>[3x]MKTIKDRIAKWSAIGLLSAVAATAFYAPSASAHGEKSQAAFMRMRTIHWYDLSWSKEKVKINETVEIKGKFHVFEGWPETVDEPDVAFLNVGMPGPVFIRKESYIGGQLVPRSVRLEIGKTYDFRVVLKARRPGDWHVHTMMNVQGGGPIIGPGKWITVEGSMSEFRNPVTTLTGQTVDLENYNEGNTYFWHAFWFAIGVAWIGYWSRRPIFIPRLLMVDAGRADELVSATDRKVAMGFLAATILIVVMAMSSANSKYPITIPLQAGTMRGMKPLELPAPTVSVKVEDATYRVPGRAMRMKLTITNHGNSPIRLGEFYTASVRFLDSDVYKDTTGYPEDLLAEDGLSVSDNSPLAPGETRTVDVTASDAAWEVYRLSDIIYDPDSRFAGLLFFFDATGNRQVVQIDAPLIPSFM;>[3x]MSAAQSAVRSHAEAVQVSRTIDWMALFVVFFVIVGSYHIH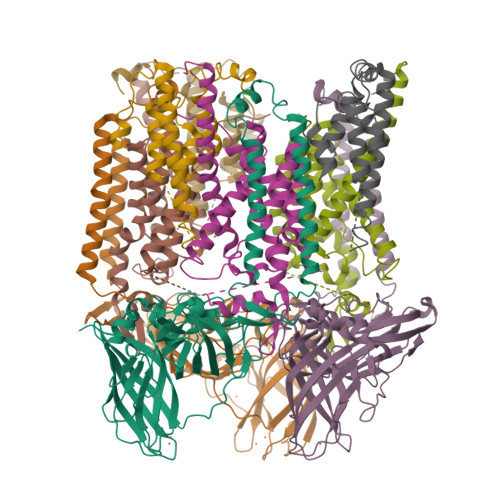AMLTMGDWDFWSDWKDRRLWVTVTPIVLVTFPAAVQSYLWERYRLPWGATVCVLGLLLGEWINRYFNFWGWTYFPINFVFPASLVPGAIILDTVLMLSGSYLFTAIVGAMGWGLIFYPGNWPIIAPLHVPVEYNGMLMSIADIQGYNYVRTGTPEYIRMVEKGTLRTFGKDVAPVSAFFSAFMSILIYFMWHFIGRWFSNERFLQST;>[3x]MAATTIGGAAAAEAPLLDKKWLTFALAIYTVFYLWVRWYEGVYGWSAGLDSFAPEFETYWMNFLYTEIVLEIVTASILWGYLWKTRDRNLAALTPREELRRNFTHLVWLVAYAWAIYWGASYFTEQDGTWHQTIVRDTDFTPSHIIEFYLSYPIYIITGFAAFIYAKTRLPFFAKGISLPYLVLVVGPFMILPNVGLNEWGHTFWFMEELFVAPLHYGFVIFGWLALAVMGTLTQTFYSFAQGGLGQSLCEAVDEGLIAK> MPSYLSPGVYVEEVASGSRPIEGVGIEGVGTSVAAFVGLAPTGPLNEPTLVTNWTQYVAAFGDFTGGYYLAHSVYGFFNNGGSAAYVVRVGGSAEDAAADGSVNGAAAPAAVTGSTAKALPAAEPKQLGTFAVTATAAGQSGPLTVEVADPEGEGPAERFKLIVKDGDKPVETFDVSAKKGNRSYVVTQVKERSKLITVTEAAPSAQLVRPENQSLTLPAPPSAAPAVPAGQAESAHPG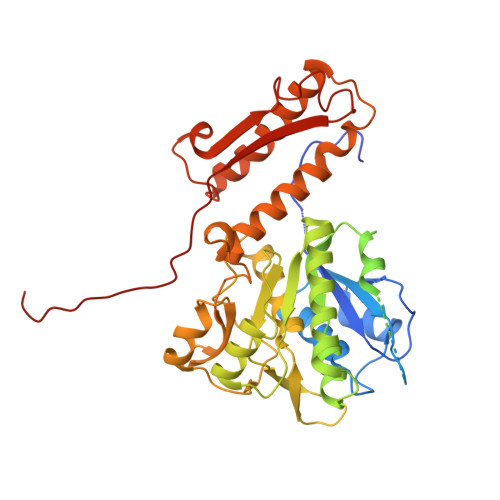PAQYLGDSSDRTGFGGLEAIDEISMVAVPDLMAAYQRGAIDLEAVKAVQLGLIAHCELMGDRVAIIDPPPNQNARQIRVWRQETAGYDSKYAALYYPWIKSFDPATGQSRLVPPSGHVAGIWARNDSERGVHKAPANEVVRGAVDLELQITRGEQDLLNPIGVNCIRSFPGRGIRVWGARTLSSDPAWRYLNIRRYFNYLEESILIGTQWVVFEPNDHNLWARIRRNVSAFLVNEWRNGALFGQSPDQAYYVKCDEETNPPESVDLGRVVCEIGIAPVKPAEFVIFRLAQFSSGGGELDE>MKKRLTESQFQEAIQGLEVGQQTIEIARGVLVDGKPQATFATSLGLTRGAVSQAVHRVWAAFEDKNLPEGYARVTAVLPEHQAYIVRKWEADAKKKQET[3x];> MKKRLTESQFQEAIQGLEVGQQTIEIARGVLVDGKPQATFATSLGLTRGAVSQAVHRVWAAFEDKNLPEGYARVTAVLPEHQAYIVRKWEADAKKKQETKR

Gene expression in the IncP-1 plasmids is stringently controlled by a network of four global repressors, KorA, KorB, TrbA and KorC interacting cooperatively. KorA is a 101-amino acid, homodimeric, protein with an N-terminal DNA-binding domain (DBD), containing a helix-turn-helix motif, and a C-terminal dimerization region, joined by a linker of four amino acids. In this study, we have determined the structures of the free KorA repressor and two complexes each bound to a 20-bp palindromic DNA duplex containing its consensus operator sequence. The structure of KorA consists of two domains, joined by a highly flexible, four amino acid linker, which retains its mobility even when bound to DNA.

The crystals of free KorA contained two dimers in the asymmetric unit (ASU), each with two N-terminal DNA Binding Domains with four α-helices and a C-Terminal Dimerization domain containing a single β-strand and the final helix from each monomer. The NOEs correlate with the X-ray crystallographic B factors for the protein and confirm that the linker is flexible. The structure of each domain is well-determined from the NMR data, and is consistent with the crystal structures. The structures of the DBD (residue 6–66) from both techniques fit with an RMSD of 0.92 Å, while the CTD structures (residues 71–98, dimer) fit with an RMSD of 2.9 Å. When the protein is removed from the DNA complex, the DBDs collapse towards each other, giving additional fluctuating contacts which keep the protein compact. Dynamic interactions observed between the two DBDs include salt bridges between R57 and E18 and hydrogen bonds between R48 and Q11/Q15. The mobility of the KorA DBDs, in the absence of DNA, is likely to be due in part to the different possible electrostatic interactions between the two domains, giving rise to multiple conformers of similar energy.>MSLVVFPFKHEHPEVLLHNVRVAAAHPRVHEVLCIGYERDQTYEAVERAAPEISRATGTPVSVRLQERLGTLRPGKGDGMNTALRYFLEETQWERIHFYDADITSFGPDWITKAEEAADFGYGLVRHYFPRASTDAMITWMITRTGFALLWPHTELSWIEQPLGGELLMRREVAAMLYEDERVRRRSDWGIDTLYTFVTVQQGVSIYECYIPEGKAHRLYGGLDDLRTMLVECFAAIQSLQHEVVGQPAIHRQEHPHRVPVHIAERVGYDVEATLHRLMQHWTPRQVELLELFTTPVREGLRTCQRRPAFNFMDEMAWAATYHVLLEHFQPGDPDWEELLFKLWTTRVLNYTMTVALRGYDYAQQYLYRMLGRYRYQAALENGRGHPV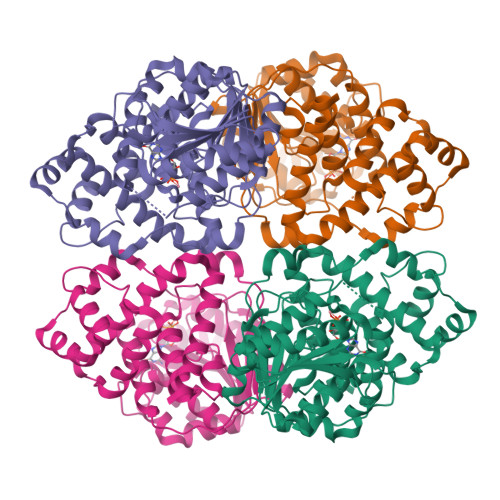PPRAALSTA[10x]Phytoglobins (Pgbs) are plant-originating heme proteins of the globin superfamily with varying degrees of hexacoordination. Pgbs have a conserved cysteine residue, the role of which is poorly understood. Class 1 Pgbs are distinguished by a weak hexacoordination (KH ≈ 2) compared to Class 2 Pgbs (KH ≈ 100). Due to the very high O2 avidity of Class 1 Pgbs, these proteins generate a tight and slow binding of O2 well suited for O2-dependent nitric oxide (NO) scavenging in low O2-containing environments.

In this comparative study, we investigated the role of Cys86 in BvPgb1.2 by generating an alanine-substituted mutant. The imposed substitution did not affect the overall tertiary structure, but led to significantly faster autoxidation rates and a minor increase in thermal stability. However, the overall 3D structures were very similar. The main differences can be found in the helical arrangement of the F-helix. In the WT, this helix starts with a Glu residue, while, in the mutant, the helix seems shorter and starts two positions downstream with a Ser residue. As a result, the direction of the side-chains has different orientations as clearly observed in the proximal His, which is almost in a perpendicular position compared to the proximal His in the WT. In helix E, where the mutation was located, no apparent differences could be observed compared to the helix E in the WT. Even though this possibility cannot be dismissed for BvPgb1.2, it is evident that the substituted cysteine did not contribute to increased monomer content. The redox balance is altered when the cysteine is removed, reducing the ability of the heme to stay in its active ferrous form. Thus, since the oxidative state of Cys86Ala is pushed toward the inactive ferric state, fewer radicals are formed in the reaction with the peroxide, ultimately leading to less activation of the possible substrates in the peroxidase reaction.

>[2x]MSFTNVNYPASDGTVIFTEEQEALVVQSWNVMKKNSAELGLKLFLKIFEIAPTAKKMFSFVRDSDVPLEQNQKLKGHAMSVFVMTAKSAAQLRKAGKVTFGESSLKHMGSVHLKYGVVDEHFEVTRFALLETIKEAVPEMWSPEMKNAWAEAFNHLVAAIKAEMQRLSTQP> ARTXQT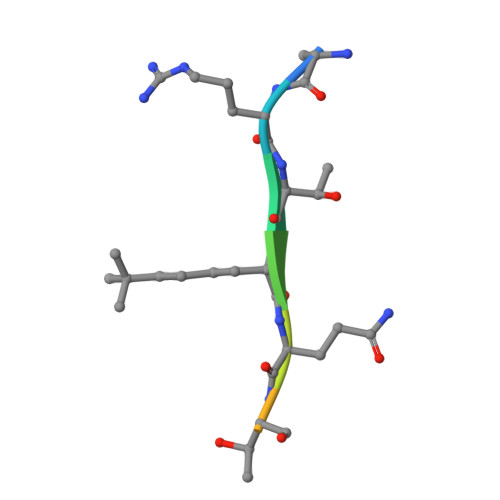ARKS>[2x]MSQVSTEFIPTRIAILTVSNRRGEEDDTSGHYLRDSAQEAGHHVVDKAIVKENRYAIRAQVSAWIASDDVQVVLITGGTGLTEGDQAP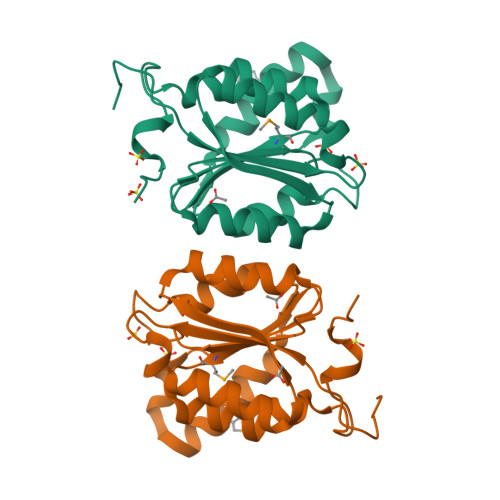EALLPLFDREVEGFGEVFRMLSFEEIGTSTLQSRAVAGVANKTLILAMPGSTKACRTAWENIIAPQLDARTRPCNFHPHLKKGS> ATALAEMPKRKFTIDDFDIGRPLGKGKFGNVYLAREKQNKFIMALKVLFKSQLEKEGVEHQLRREIEIQSHLRHPNILRMYNYFHDRKRIYLMLEFAPRGELYKELQKHGRFDEQRSATFMEELADALHYCHERKVIHRDIKPENLLM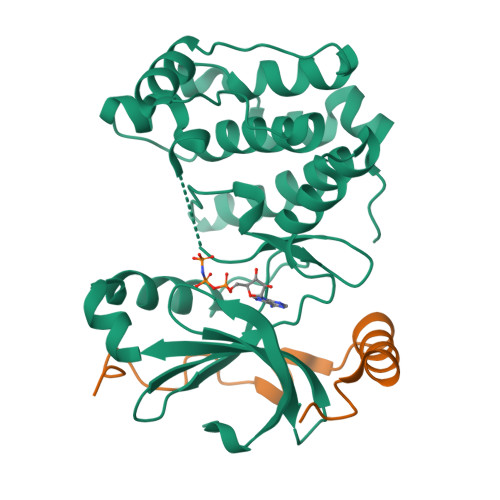GYKGELKIADFGWSVHAPSLRRRTMCGTLDYLPPEMIEGKTHDEKVDLWCAGVLCYEFLVGMPPFDSPSHTETHRRIVNVDLKFPPFLSDGSKDLISKLLRYHPPQRLPLKGVMEHPWVKANSRRVLPGVYQSTQSKD;> PIPAWASGNLLTQAIRQQYYKPIDVDRMYGTIDSPKLEELFNKS>[2x]METKDLIVIGGGINGAGIAADAAGRGLSVLMLEAQDLACATSSASSKLIHGGLRYLEHYEFRLV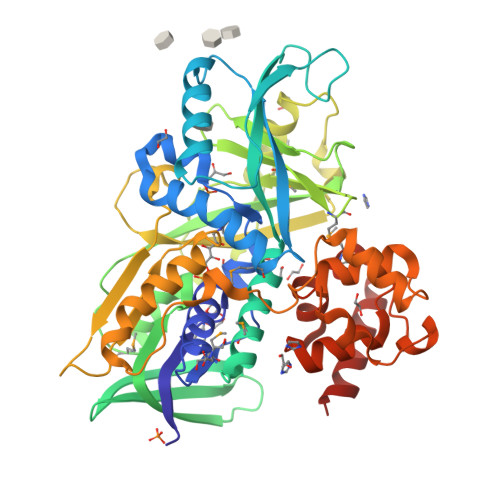SEALAEREVLLKMAPHIAFPMRFRLPHRPHLRPAWMIRIGLFMYDHLGKRTSLPGSTGLRFGANSVLKPEIKRGFEYSDCWVDDARLVLANAQMVVRKGGEVLTRTRATSARRENGLWIVEAEDIDTGKKYSWQARGLVNATGPWVKQFFDDGMHLPSPYGIRLIKGSHIVVPRVHTQKQAYILQNEDKRIVFVIPWMDEFSIIGTTDVEYKGDPKAVKIEESEINYLLNVYNTHFKKQLSRDDIVWTYSGVRPLCDDESDSPQAITRDYTLDIHDENGKAPLLSVFGGKLTTYRKLAEHALEKLTPYYQGIGPAWTKESVLPGGAIEGDRDDYAARLRRRYPFLTESLARHYARTYGSNSELLLGNAGTVSDLGEDFGHEFYEAELKYLVDHEWVRRADDALWRRTKQGMWLNADQQSRVSQWLVEYTQQRLSLAS> ATCYCR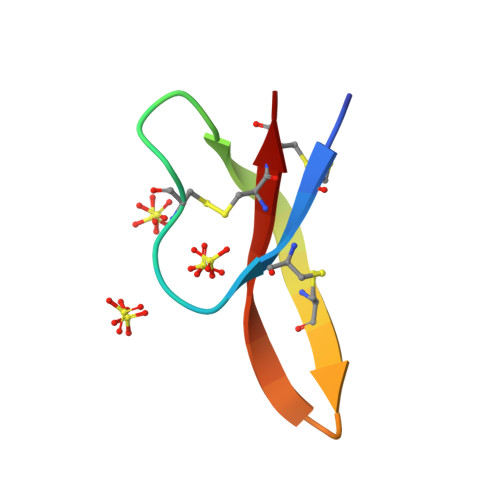TGRCATRESLSGVCRISGRLYRLCCR>[8x]SMRLSDIETFVVGNPPPRHGGRYFIFVKLVTACGITGYGEIYNATFGPDLVAKMAEDVFARQFAGEDPHHIEKLWHKTYGAGYTQRPDVTVMGVLSGLEMACWDIIGKAAGKPAYELLGGKVHERLRSYTYLYPTDGDVYPDPDKPNVYNDADMAAEAAAKAVDQGFTAVKFDPAG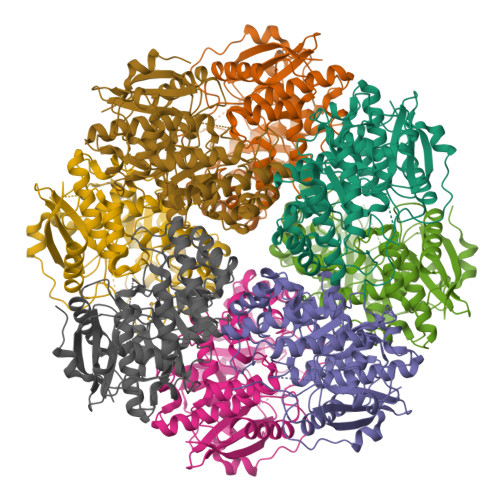AYTIYDGHQPSLEDLERSEAFCKQIRAAVGTKADLLFGTHGQFTVSGAKRLARRLEAYDPLWFEEPIPPEKPEDMAEVARYTSIPVATGERLCTKYEFSRVLETGAASILQMNLGRVGGLLEAKKIAAMAECHSAQIAPHLYCGPLVALANIQLATCSPNFLVLESIRTFDGFFAELLTTPIRWENGYIIPSQEPGLGHDLNEDVARANPYTGSDLHLGFQETPALPL> RSAFSKIESEEYNSLKSSTIQTIGTSDGGSGIGYIESGDYLVFNKINF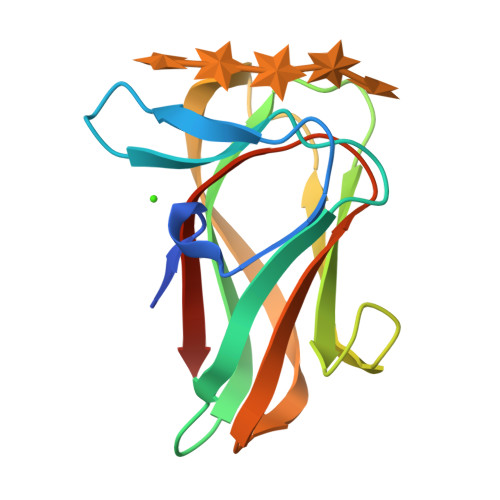GNGANSFKARVASGADTPTNIQLRLGSPTGTLIGTLTVASTGGWNNYEEKSCSITNTTGQHDLYLVFSGPVNIDYFIFDSNGVNP> ADDIVLKAENGDVKFPHKA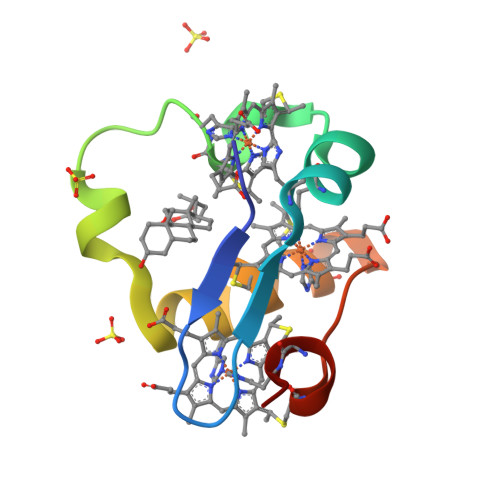HQKAVPDCKKCHEKGPGKIEGFGKEMAHGKGCKGCHEEMKKGPTKCGECHKK>[2x]GTD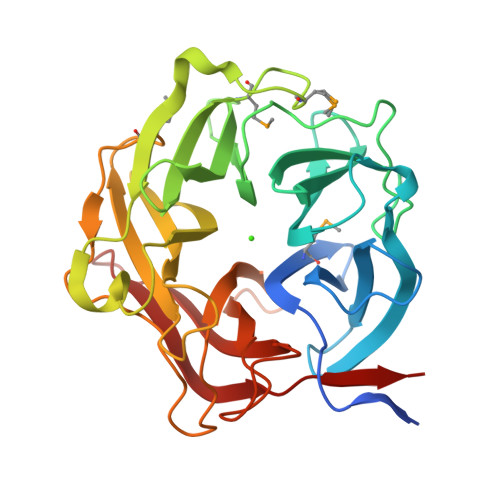DEEKDNNGQGSVSVETNYLPIADPYVMFYNNKYYAYGTGGTTAGEGFACFSSDDLKNWKREGQALSATDSYGTWGFWAPEVYYVESKKKFYLFYSAEEHICVATSTTPEGPFRQEVKQPIWSEKSIDTSLFIDDDGTPYLYFVRFTDGNVIWVAQMTDDLMSIKTETLNQCIKAEVSWELLQGKVAEGPSLLKKNGVYYLIYSANHYENKGYGVGYATSDTPMGPWVKYSKNPLLQGDAATGLVGTGHGAPFQCKDGSWKYIFHAHWSAAEIQPRTSYIKDFAISDQGVVTISGTVIKPRVLK> GSHMEILWNEAKAFIAECYQELGKEEEVKDRLDSIKSEIDRTGSYVHTKEELEHGAKMAWRNSNRCIGRLFWNSLNVIDRRDVRTKEDVRDALFHHIETATNNGKIRPSITIFPPEEKGEKQVEIWNHQLIRYAGYEGERIGDPASRSLTAACEQLGWRGERTDFDLLPLIFRMRGDEQPVWYELPRSLVIEVPITHPDIEAFSDLELKWYGVPIISDMKLEVGGIHYNAAPFNGWYMGTEIGARNLADEKRYDKLKKVASVIGISTNYNTDLWKDQALVELNKAVLYSYKKQGVSIVDHHTAASQFKRFEEQEEEAGRKLTGDWTWLIPPISPAATHIFHRSYDNSIVKPNYFYQ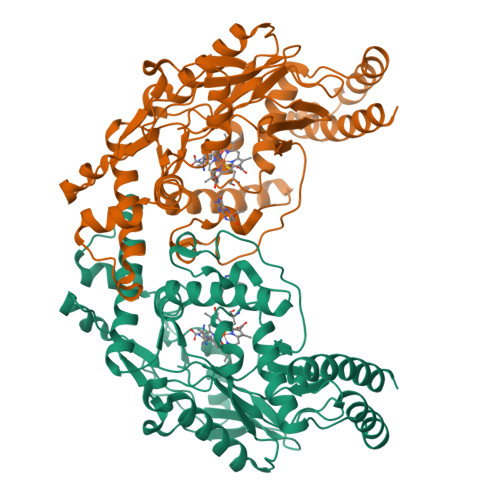DKPYE> MSESLSWMQTGDTLALSGELDQDVLLPLWEMREEAV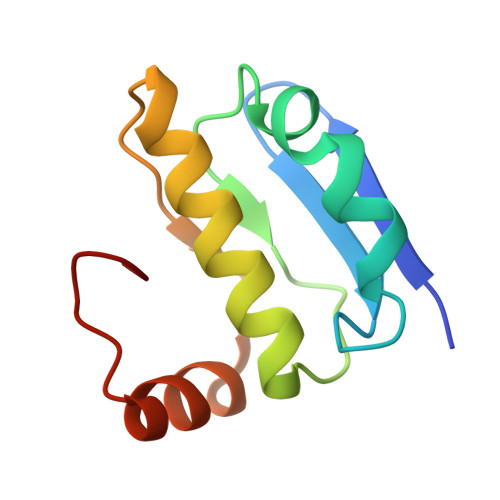KGITCIDLSRVSRVDTGGLALLLHLIDLAKKQGNNVTLQGVNDKVYTLAKLYNLPADVLPR> MDALQMAVGYFEKGPIKASQNKDKTLEKHLKTVENVAWKNGLASEEIDILLNIALSGKFGNAVNTRILKCMIPATVISEDSVVKAVSWLCVGKCSGSTKVLFYRWLVAMFDFIDRKEQINLLYGFFFASLQDDALCPYVCHLLYLLTKKENVKPFRVRKLLDLQAKMGMQPHLQALLSLYKFFAPALISVSLPVRKKIYFKNSENLWKTALLAVKQRNRSPLE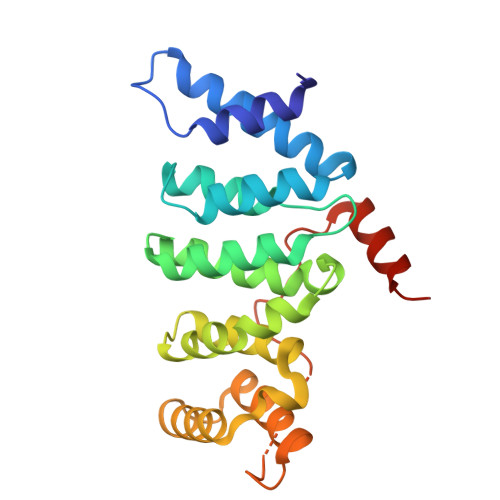VQFG>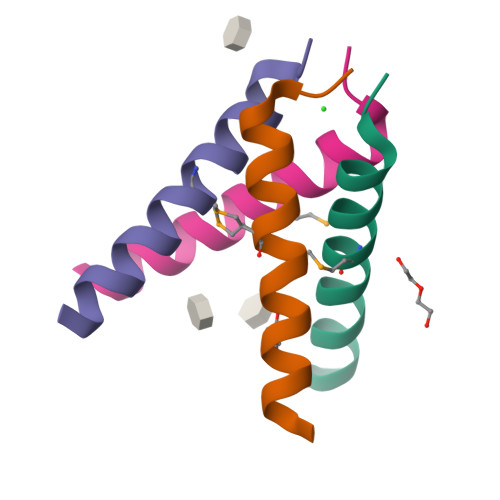[8x]SSDPLVVAASIMGILHLILWILDRLX> MTAVVKNLAKLPAATSQILTNVSKLQTFHGLLEERRDKYAPLAYHTYDNLKQKTTWHPIAHAWVDEGLPVSKKEYNEYCWLKKDMQRLLPLASPFVFGIYGILPLAVWLSNDGYLPSAFSSKKDIVSKKLEWYSSYGDDLRQQVGPMLQHRLKRHLRGTLNNEHRLMLDEVTESYKEIFYSHYTGQLRDVRKCAHLRLYDGTSTVLLLTNKEPVELTSELLQKWNAIKAAKLSPEEEKKARNEALIEAYKEQELHGGPHVKHMQGYGIPSDTPLLGENAKGDQYTQPPESASIPLEQLEWTGDTVFIPAEYRTEVEDWGRELTKLANQFLLLPWRFVSNAWNQRRLVSWFEEILQEDALIAKEGGVQALSDDELKVALLDRAVIRCDEELTRGDMEARYKEISWLMSLRNPFIVLAWQTGYYRSTYSPEDDLPEASILPKLNRTVLDVDVHNELAPDHPEKPLPRVHPALYPNSHLALAKEVAVLAK;> MAAKTIPFVASTALGERLFAGVQKVLAAAKAPVSLVQTDAKFAPADAKYLLAEPLSAAATGELANKYGLSSKVTSGAASQFYPNSIYPSLNVEVVQNLYALSNPAFSSLSATTTKAVTV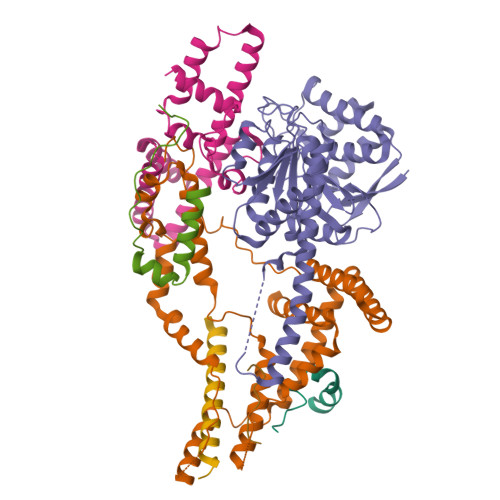KDESAIKLAELQKETERNISSFFRDEANKSVQATLRLACDKAIKTKADKKTVMVVTKPHGDAFDDLLAQVTKSESDGRADELRNSSVSVEPTLVGNAWPKLVMFPEGVNVVVCGPNASGDQVAQLFVGIAGGTGMVAQQLVGDAVVFTSANAEDNENPTGALLAASNLLTALGHEAEAKKIAAAVAKAYTTDRILPKELPGGKADLEAFIDAVAKHASA;> MFRGFRPVLAADAVKFQTLYNVLTGKQHLKDQVPVKDCNLTAIFGASWKADLNKWFDSEYAPKLPAAERDSAKKSLDLYLKRVDLTRYTREELTTYGILACGPGKVDALTEKHLLETGKARLEELTAGLGNKDEGVNAFRKEVEQEGKYANWPAEKSKALADKVIAASP;> MMRRACRIIRPSHVRGVSGVAPTIYLRSKAALPATSTTDVRPQLYALQRFAKAQLKTATEAERAAIEADIARYQEYLDSDLEKLKQDVAEDTAKKQKLIPLLDRYPDVPIEKIPEHANVLLKKIDACLEILSKDIGEVTDAEAHEMYFETSKFQILHIYTGCVASFPEGDVPPGAVECLPGQVIRTKVNGEDVMLEIDEVDPGYQVCWFKPDVPLPENAEILWSYPYEPTAALPTGTTWEEGQANVLIPAEPTPEAAVWPPTPVTNVYAPMAEKLALKSNPELKVLFKEALLQPAKLLPLDVDYQCSHDREVVEAKRDRYLTALVEAEQAPPLPFTPDVLQLQLEHNVLKGELIDRLRALEYTIVTEQLQARLHERRLRGDVIDEWEELDYHPLVRDDTYLAIDFGDPTFGRYIWKLFPHTDGDEECMFKDTRLDVLPPQVNPLNAILAQHTAQTPVHRSLEKRLWTEVRATAVSE;> MHMRRAVSVFGRCRSLNGLRNYAVPSPKYIEIYQSDFSRNAYPLELLGGSHVDFAKLLYSFADQVENKKFEVYVEDFKKLDSIIAEKGPFWAEEKIFQSPTFQGLSEGFKFILGWIQSEGAIDRLENVRLAYKELVNEARKETTATVIVAKEPSGNDLAEIRKQVEELHKESPLKDYKLVLETKVDPSIGGGYILEVCNQVVNRSAAAAAAETAALAKASAAQVDWTSLPAAPPRPSPSAPDTLIRLLGSVVDDLADADKVEQKYGA;> MPSTSPADKDVPMSILHTHGLSYVNWCMSLAPGLLVFEGFFRARYYRSRVPPSRTVLMNGLKMRMFSLARQQAPKIVHKPVLSPIPEHLRLVKNVAQVQIDMLKLLNAQAAK;> LIPVSLVDLININIIFYILLLYTLLLFFIPLFLASINYTYHYIYKYYNYNYNFINNNT> MSEYMDDVDREFINCLFPSYLLQQPVAYDLWILYLQHRKLFHKLKNTNLINADENPTGVGMGRTKLTALTRKEIWSKLMNLGVLGTISFEAVNDDYLIQVYKYFYPDVNDFTLRFGVKDSNKNSVRVMKASSDMRKNAQELLEPVLSEREMALNSNTSLENDRNDDDDDDDDDDDDDDDDDDDDDESDLESLEGEVDTDTDDNNEGDGSDNHEEGGEEGSRGADADVSSAQQRAERVADPWIYQRSRSAINIETESRNLWDTSDKNSGLQYYP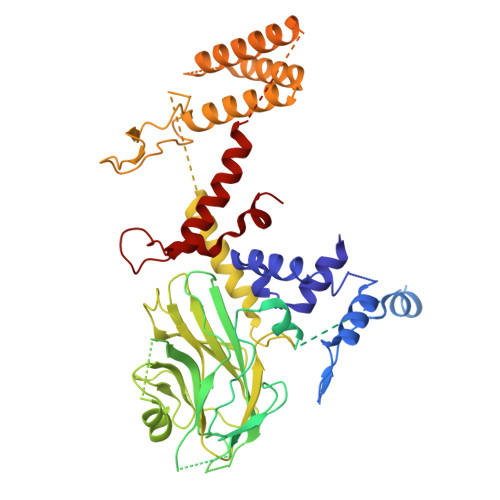PDQSPSSSFSSPRVSSGNDKNDNEATNVLSNSGSKKKNSMIPDIYKILGYFLPSRWQAQPNNSLQLSQDGITHLQPNPDYHSYMTYERSSASSASTRNRLRTSFENSGKVDFAVTWANKSLPDNKLTIFYYEIKVLSVTSTESAENSNIVIGYKLVENELMEATTKKSVSRSSVAGSSSSLGGSNNMSSNRVPSTSFTMEGTQRRDYIYEGGVSAMSLNVDGSINKCQKYGFDLNVFGYCGFDGLITNSTEQSKEYAKPFGRDDVIGCGINFIDGSIFFTKNGIHLGNAFTDLNDLEFVPYVALRPGNSIKTNFGLNEDFVFDIIGYQDKWKSLAYEHICRGRQMDVSIEEFDSDESEEDETENGPEENKSTNVNEDLMDIDQEDGAAGNKDTKKLNDEKDNNLKFLLGEDNRFIDGKLVRPDVNNINNLSVDDGSLPNTLNVMINDYLIHEGLVDVAKGFLKDLQKDAVNVNGQHSESKDVIRHNERQIMKEERMVKIRQELRYLINKGQISKCINYIDNEIPDLLKNNLELVFELKLANYLVMIKKSSSKDDDEIENLILKGQELSNEFIYDTKIPQSLRDRFSGQLSNVSALLAYSNPLVEAPKEISGYLSDEYLQERLFQVSNNTILTFLHKDSECALENVISNTRAMLSTLLEYNAFGSTNSSDPRYYKAINFDEDVLNL>[60x]GGGVGVSTGSYDNQTHYKFLGDGWVEITAYSTRMVHLNMPKSENYCRVRVHNTNDTGTASHMAMDDAHEQIWTPWSLVDANAWGVWFQPSDWQYISNNMIHINLHSLDQELFNVVIKTVTEQNTGAEAIKVYNNDLTAAMMVALDSNNILPYTPAIDNQETLGFYPWKPTIPSPYRYYFSCDRNLSVTYKDEAGTITDTMGLASGLNSQFFTIENTQRINLLRTGDEYATGTYYFDTEPIRLTHTWQTNRHLGQPPQITELPSSDTANATLTARGYRSGLTQIQGRNDVTEATRVRPAQVGFCQPHDNF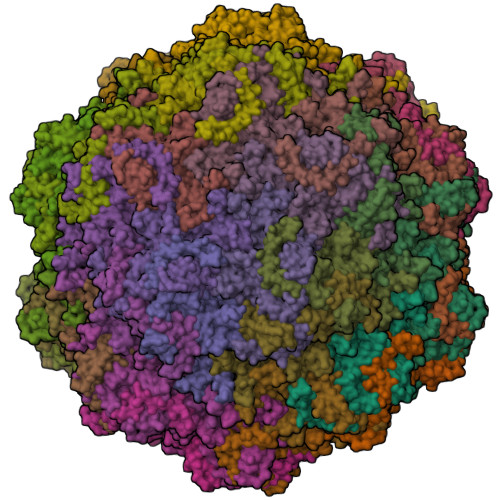ETSRAGPFKVPVVPADITQGLDHDANGSLRYTYDKQHGQSWASQNNKDRYTWDAVNYDSGRWTNNCFIQSVPFTSEPNANQILTNRDNLAGKTDIHFTNAFNSYGPLTAFPHPAPIYPQGQIWDKELDLEHKPRLHTQAPFVCKNNAPGQLLVRLAPNLTDQYDPNSSNLSRIVTYGTFFWKGKLTLKAKMRPNATWNPVFQISATNQGTNDYMSIERWLPTATGNITNVPLLSRPVARNTY>[2x]MERTFVMIKPDGVRRGLVGEILARFERKGFRIAALKLMQISQELAERHYAEHREKPFFPGLVRFITSG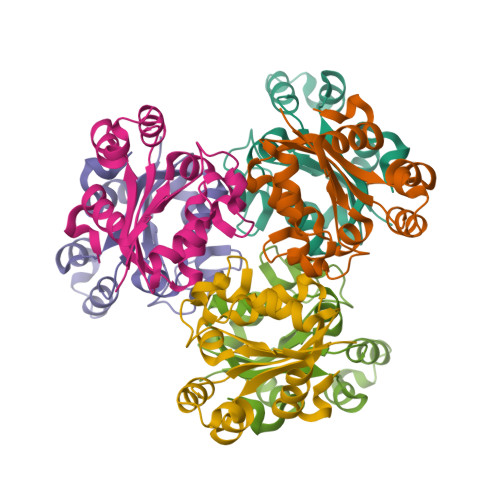PVVAMVLEGPGVVAEVRKMMGATHPKDALPGTIRGDFATTIDENVIHGSATLEDAQREIALFFRPEELL As a key mitochondrial Ca2+ transporter, NCLX regulates intracellular Ca2+ signalling and vital mitochondrial processes. Here we report the cryogenic electron microscopy (cryo-EM) structures of rat NCLX in cytosol-facing (intermembrane space) and matrix-facing conformations, with and without Ca2+. Each NCLX protomer contains twelve transmembrane helices and two sets of helical hairpins/bundles roughly parallel to the membrane. The structure comprises a transport domain, which mediates NCLX trimer formation at the centre, and a gate domain, located on the periphery without contacting other protomers.

Under Ca2+-free conditions, we also observed distinct assemblies, including all three protomers in matrix-facing; one or two in cytosol-facing; or all three in cytosol-facing conformation. By contrast, the structure determined at pH 7.4 without Ca2+ displays a combination of cytosol- and matrix-open, or all matrix-open, conformations within a trimer, compatible with NCLX potentially in mixed protonated states. Moreover, no obvious Na+ ion densities were observed in NCLX structures solved with 150 mM Na+ under Ca2+-free conditions (at the same pH of 7.4), raising the possibility that Na+ is a poor ligand for NCLX. NCLX exhibits similar overall structures with and without Ca2+ (both at pH 7.4). In the matrix-facing conformation, the Ca2+-bound and -free structures superimpose well. In the matrix-facing conformation, a cavity opens to the matrix and extends to near the membrane centre. This cavity is mainly lined by TM2, TM8, TM9, part of TM3, and the loop between α2 and α3. The highly tilted TM1 and TM8 (within the gate domain) interact with TM2 and TM9 (within the transport domain), respectively, blocking cytosolic access to the substrate translocation pathway mainly by the interacting F122TM1–L145TM2 residue pair, as well as the side chains of I433TM8 and N434TM8.

>[3x]MAGRWLDPLWAPGFLCVALILETASGAGDLSTKAHGHIQFSARGVNQTAMADCRAVCSLNTSDRCDFVKRNPDCHSEGGYLDYLKGIFCYFPPNLLPLAITLYVFWLLYLFLILGVTAAKFFCPNLSAISTSLKLSHNVAGVTFLAFGNGAPDIFSALVAFSDPRTAGLAIGALFGAGVLVTTVVAGGITILRPFMAASRPFLRDITFYMVAVFLTFTALYLGRITLVWALGYLGLYVFYVVTVIICTWVYQRQRSRSLVHSISETPELLTDSEEDQMSSNTNSYDYGEEYRPLLLGEETTGQILLQALNPLDYRKWRTQSISCKLLKVAKLPVEFLLLLTVPVVDPDKDDRNWKRPLNCLQLVISPLVLVLTLQSGVYGIYEIGGLLPVWAVVVIVGTALASVTFFATSNSEPPRLHWLFAFLGFLTSALWINAAATEVVNILRSLGVVFRLSNTVLGLTLLAWGNSIGDAFSDFTLARQGYPRMAFSACFGGIIFNILVGVGLGCLLQIVRSHASEVKLEPDGLLVWVLASALGLSLVFSLVSVPLQCFQLSKAYGLCLLLFYICFIVVVLLTEFGVIHLKAD>GSHMSNTQTVLPFTGLNTPSGVAVDSAGTVYVTDHGNNRVVKLAAGSNTQTVLPFTGLNTPSGVAVDSAGTVYVTDHGNNRVVKLAAGSNTQTVLPFTGLNTPSGVAVDSAGTVYVTDHGNNRVVKLAAGSNTQTVLPFTGLNTPSGVAVDSAGTVYVTDHGNNRVVKLAAGSNTQTVLPFTGLNTPSGVAVDSAGTVYVTDHGNNRVVKLAAGSNTQTVLPFTGLNTPSG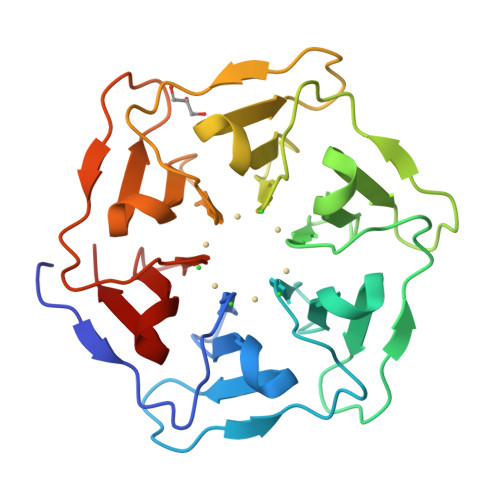VAVDSAGTVYVTDHGNNRVVKLAAG[2x]>[2x]DRHHHHHHGSEVVVEWSRDQYHVLFDSYRDNVAGKSFQTRLCLPMPIDVVYTWVNGTDPKL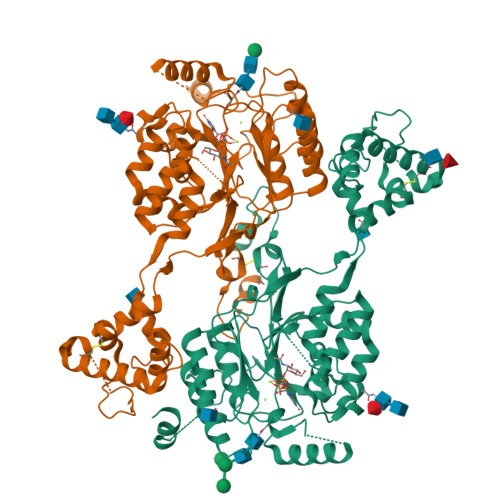IKEVTELKRSKRDPLIPECQGKQTPEKDKCYRDDNTASRFEDNEELRYSLRSIEKHAPWVRHIFIVTNGQIPSWLNLDNPRVSVVTHQDIFQNQTHLPTFSSPAIETHIHRIPGLSQKFIYLNDDVMFGKDVWPDDFYSHSKGQKVYLTWPVPNDTFADSLRYVNRLLNAQFGFTSRKVPAHMPHMIDRLIMQELQDTFPQEFDKTSSHRVRHSEDMQFAFSYFYFLMSAVQQLNISEVFDEIDTDHSGVLSDREIRTLATRIHELPLSLQDLTSLEQMLINCSKSLPSNLTHLHAVSPTQEAYYDPSMPPVTKGLVIHCKPITERIHKAFKDQNKYKFEIMGEEEIAFKMIRTNVSHVVGQLDDIRKNPRKFICLNDNIDHIHKDAGTVKAVLRDFYESMFPLPSQFELPREYRNRFLHMTELQEWRIYRDKL> MDYKDDDDKRSPVRDLARNDGEESTDRTPLLPGAPRAEAAPVCCSARYNLAILAFFGFFIVYALRVNLSVALVDMVDSNTTLEDNRTSKACPE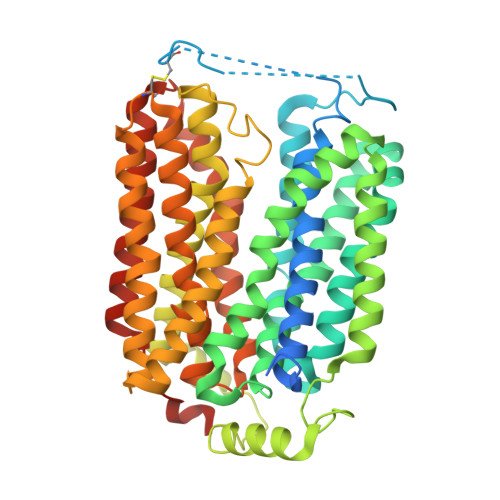HSAPIKVHHNQTGKKYQWDAETQGWILGSFFYGYIITQIPGGYVASKIGGKMLLGFGILGTAVLTLFTPIAADLGVGPLIVLKALEGLGEGVTFPAMHAMWSSWAPPLERSKLLSISYAGAQLGTVISLPLSGIICYYMNWTYVFYFFGTIGIFWFLLWIWLVSDTPQKHKRISHYEKEYILSSLRNQLSSQKSVPWVPILKSLPLWAIVVAHFSYNWTFYTLLTLLPTYMKEILRFNVQENGFLSSLPYLGSWLCMILSGQAADNLRAKWNFSTLCVRRIFSLIGMIGPAVFLVAAGFIGCDYSLAVAFLTISTTLGGFCSSGFSINHLDIAPSYAGILLGITNTFATIPGMVGPVIAKSLTPDNTVGEWQTVFYIAAAINVFGAIFFTLFAKGEVQNWALNDHHGHRH> GVFPSSVYVPDEWEVSREKITLLRELGQGSFGMVYEGNARDIIKGEAETRVAVKTVNESASLRERIEFLNEASVMKGFTCHHVVRLLGVVSKGQPTLVVMELMAHGDLKSYLRSLRPE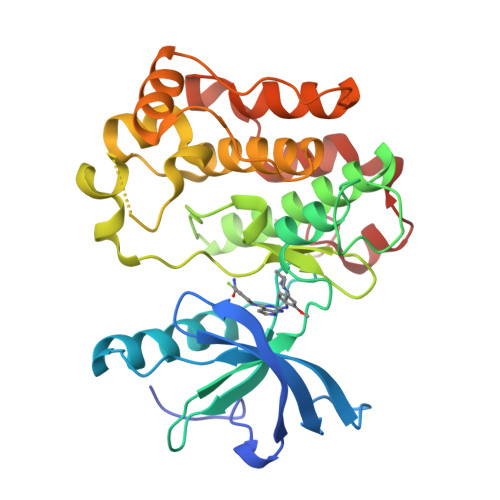AENNPGRPPPTLQEMIQMAAEIADGMAYLNAKKFVHRNLAARNCMVAHDFTVKIGDFGMTRDIYETDYYRKGGKGLLPVRWMAPESLKDGVFTTSSDMWSFGVVLWEITSLAEQPYQGLSNEQVLKFVMDGGYLDQPDNCPERVTDLMRMCWQFNPNMRPTFLEIVNLLKDDLHPSFPEVSFFHSEENK> MTATVLLEVPFSARGDRIPDAVAELRTREPIRKVRTITGAEAWLVSSYALCTQVLEDRRFSMKETAAAGAPRLNALTVPPEVVNNMGNIADAGLRKAVMKAITPKAPGLEQFLRDTANSLLDNLITEGAPADLRNDFADPLATALHCKVLGIPQEDGPKLFRSLSIAFMSSADPIPAAKINWDRDIEYMAGILENPNITTGLMGELSRLRKDPAYSHVSDELFATIGVTFFGAGVISTGSFLTTALISLIQRPQLRNLLHEKPELIPAGVEELLRINLAFADGLPRLATADIQVGDVLVRKGELVLVLLEGANFDPEHFPNPGSIELDRPNPTSHLAFGRGQHFCPGSALGRRHAQIGIEALLKKMPGVDLAV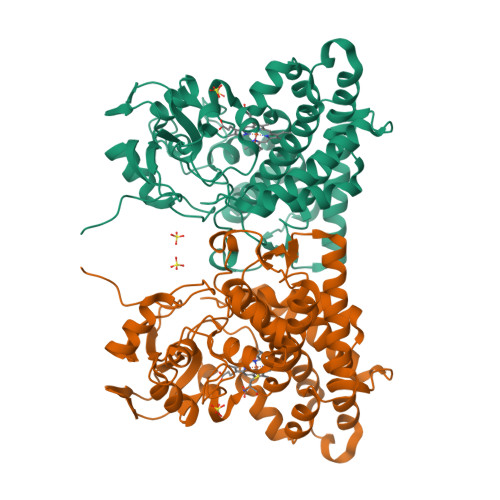PIDQLVWRTRFQRRIPERLPVLW[(5R)-5-amino-5-carboxy-8-hydroxyoctyl](trihydroxy)borate(1-) | C9 H21 B N O6 | 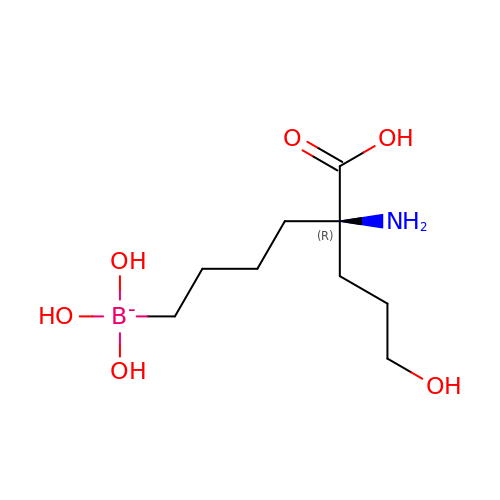NLSMSWJRKXBPCL-SECBINFHSA-N>SGPGKELPVVWAQEGAPVHLPCSLKSPNLDPNFLRRGGVIWQHQPDSGQPTPIPALDLHQGMPSPRQPAPGRYTVLSVAPGGLRSGRQPLHPHVQLEERGLQRGDFSLWLRPALRTDAGEYHATVRLPNRALSCSLRLRVGQASMIASPSGVLKLSDWVLLNCSFSRPDRPVSVHWFQGQNRVPVYNSPRHFLAETF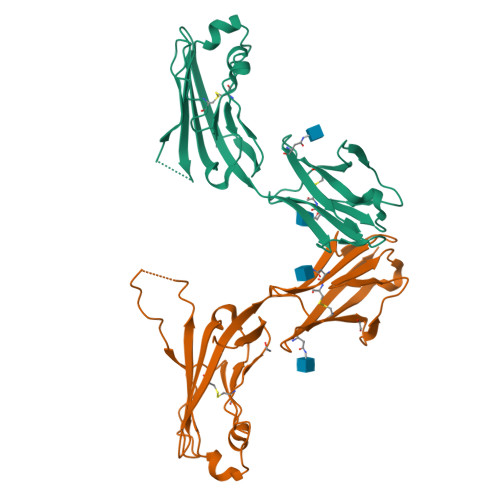LLLPQVSPLDSGTWGCVLTYRDGFNVSITYNLKVL[2x]>[2x]GVPFLTELKERFIRWLDHDNDGQSTFDEVKNYIRRFKPDVTDQTVAAFISRRDSN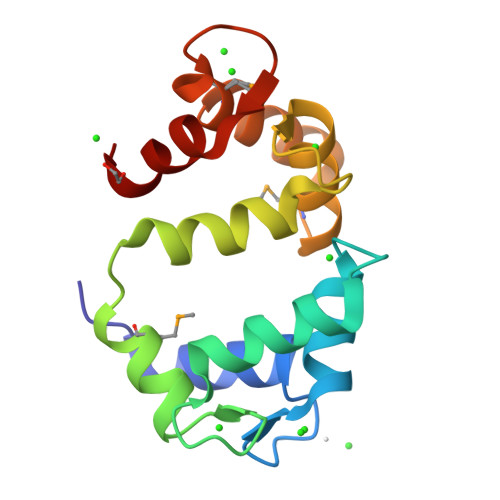GNGAIDFVPEYVHDMAAPDYTLEGANEWFKLQDTNDDSFVTEAELVKVAEAVGMSPEEALDTVQGYYMSADANKDGKLSLDEFKTLYSP3-[(4-fluorobenzyl)sulfanyl]-4H-1,2,4-triazole | C9 H8 F 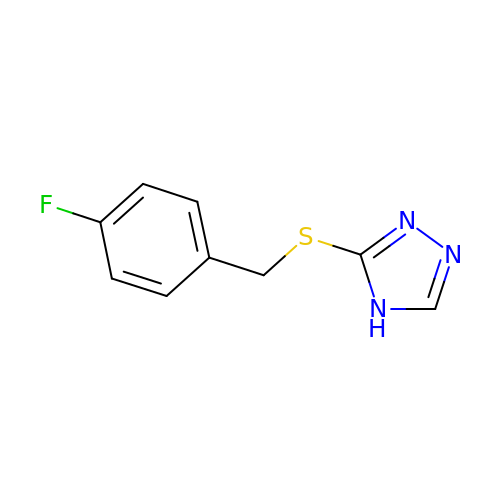N3 S | XLRSDRUBTQOPEY-UHFFFAOYSA-N ALLOXAN | C4 H2 N2 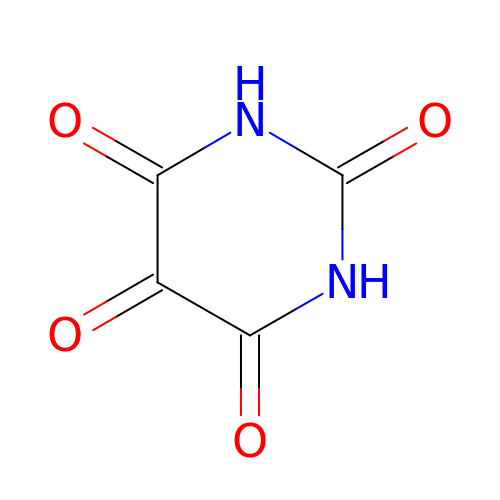O4 | HIMXGTXNXJYFGB-UHFFFAOYSA-N> MLESNENRIQIMSTIAKIYRAMSRELNRRLGELNLSYLDFLVLRATSDGPKTMAYLANRYFVTQSAITAS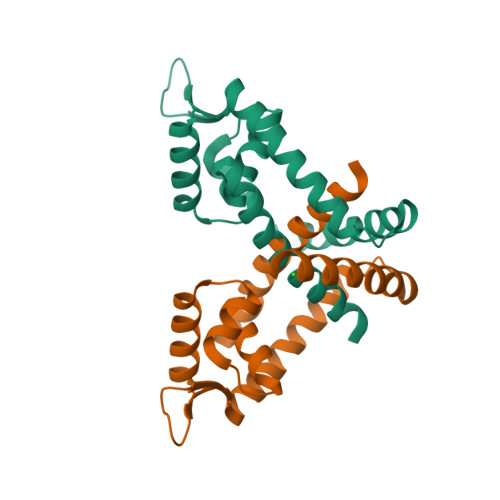VDKLEEMGLVVRVRDREDRAKILIEITEKGLETFNKGIEIYKKLANEVTGDLSEDEVILVLDKISKILKRIEEISQ5-(2-OXO-HEXAHYDRO-THIENO[3,4-D]IMIDAZOL-6-YL)-PENTANOIC ACID (4-NITRO-PHENYL)-AMIDE 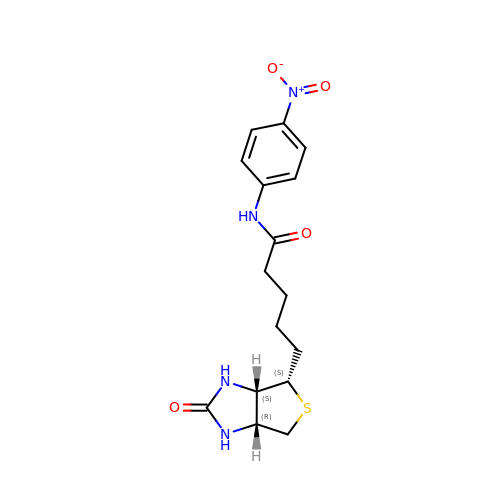| C16 H20 N4 O4 S | PORZMUYPQKOFQY-YDHLFZDLSA-N>QLTTESMPFNVAEGKEVLLLVHNLPQQLFGYSWYKGERVDGNRQIVGYAIGTQQATPGPANSGRETIYPNASLLIQNVTQNDTGFYTLQVAK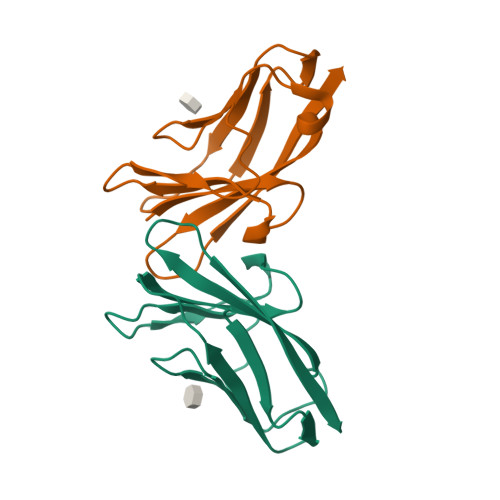SDLVNEEATGQFHVY[2x]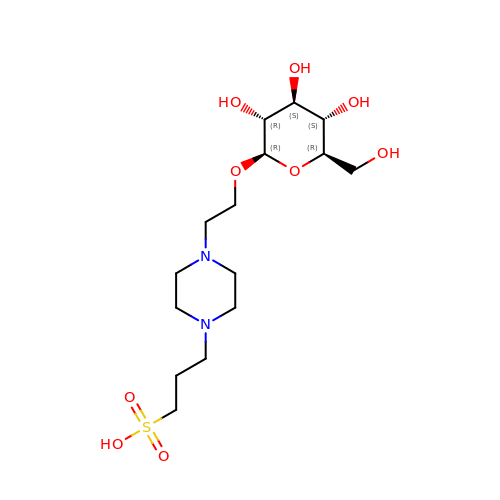3-{4-[2-(beta-D-glucopyranosyloxy)ethyl]piperazin-1-yl}propane-1-sulfonic acid | C15 H30 N2 O9 S | DAJNLGJHGLHERP-UXXRCYHCSA-N> RGSFVEMLPRETDEEPEEPGRRGSFVEMVDNLRGKSGQGYYVEMTVGSPPQTLNILVDTGS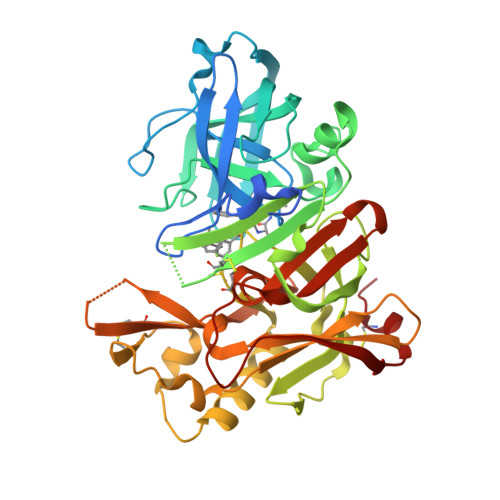SNFAVGAAPHPFLHRYYQRQLSSTYRDLRKGVYVPYTQGAWAGELGTDLVSIPHGPNVTVRANIAAITESDKFFINGSNWEGILGLAYAEIARPDDSLEPFFDSLVKQTHVPNLFSLQLCGAGFPLNQSEVLASVGGSMIIGGIDHSLYTGSLWYTPIRREWYYEVIIVRVEINGQDLKMDCKEYNYDKSIVDSGTTNLRLPKKVFEAAVKSIKAASSTEKFPDGFWLGEQLVCWQAGTTPWNIFPVISLYLMGEVTNQSFRITILPQQYLRPVEDVATSQDDCYKFAISQSSTGTVMGAVIMEGFYVVFDRARKRIGFAVSACHVHDEFRTAAVEGPFVTLDMEDCGYN> GSDLTYAYLVGLFEGDGYFSITKKGKYLTYELGIELSIKDVQLIYKIKKILGIGIVSFR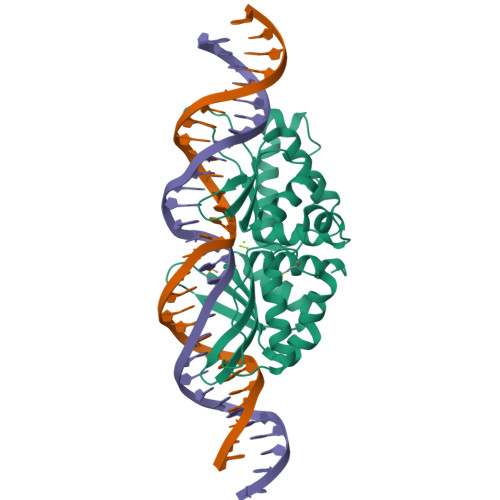KRNEIEMVALRIRDKNHLKSFILPIFEKYPMFSNKQYDYLRFRNALLSGIISLEDLPDYTRSDEPLNSIESIINTSYFSAWLVGFIEAEGCFSVYKLNKDDDYLIASFDIAQRDGDILISAIRKYLSFTTKVYLDKTNCSKLKVTSVRSVENIIKFLQNAPVKLLGNKKLQYLLWLKQLRKISRYSEKIKIPSNY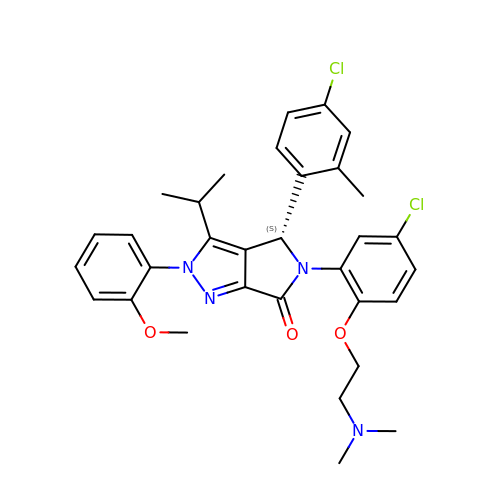(4~{S})-5-[5-chloranyl-2-[2-(dimethylamino)ethoxy]phenyl]-4-(4-chloranyl-2-methyl-phenyl)-2-(2-methoxyphenyl)-3-propan-2-yl-4~{H}-pyrrolo[3,4-c]pyrazol-6-one | C32 H34 Cl2 N4 O3 | YBMQYNARIZUNIO-HKBQPEDESA-N> MANLEKKRVVVTGLGAITPIGNTLQDYWQGLMEGRNGIGPITRFDASDQACRFGGEVKDFDATQFLDRKEAKRMDRFCHFAVCASQQAINDAKLVINELNADEIGVLIGTGIGGLKVLEDQQTILLDKGPSRCSPFMIPMMIANMASGLTAINLGAKGPNNCTVTACAAGSNAIGDAFRLVQNGYAKAMICGGTEAAITPLSYAGFASARALSFRNDDPLHASRPFDKDRDGFVMGEGSGILILEE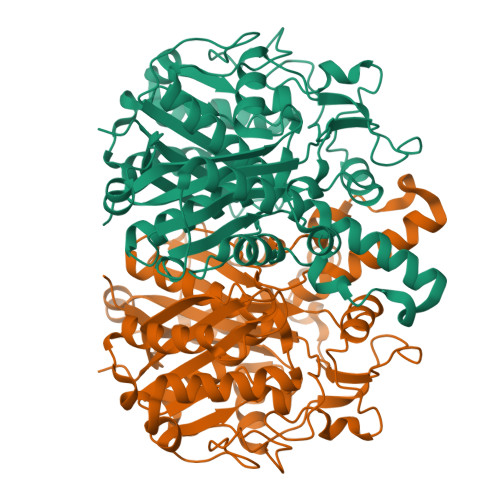LESALARGAKIYGEMVGYAMTCDAYHITAPVPDGRGATRAIAWALKDSGLKPEMVSYINAHGTSTPANDVTETRAIKQALGNHAYNIAVSSTKSMTGHLLGGSGGIEAVATVMAIAEDKVPPTINLENPDPECDLDYVPGQSRALIVDVALSNSFGFGGHNVTLAFKKYQ> MGSSHHHHHHSSGPQQGLRQPQKEETKRPNIIFMMTDDHTTQAMSCYGGNLIQTPNMDRIANEGIRFDNCYAVNALSGPSRACILTGKFSHENGFTDNASTFNGDQQTFPKLLQQAGYQTAMIGKWHLISEPQGFDHWSILSGQHEQGDYYDPDFWEDGKHIVEKGYATDIITDKAINFLENRDKNKPFCMMYHQKAPHRNWMPAPRHLGIFNNTIFPEPANLFDDYEGRGKAAREQDMSIEHTLTNDWDLKLLTREEMLKDTTNRLYSVYKRMPSEVQDKWDSAYAQRIAEYRKGDLKGKALISWKYQQYMRDYLATVLAVDENIGRLLNYLEKIGELDNTIIVYTSDQGFFLGEHGWFDKRFMYEECQRMPLIIRYPKAIKAGSTSSAISMNVDFAPTFLDFAGVEVPSDIQGASLKPVLENEGKTPADWRKAAYYHYYEYPAEHSVKRHYGIRTQDFKLIHFYNDIDEWEMYDMKADPREMNNIFGKAEYAKKQK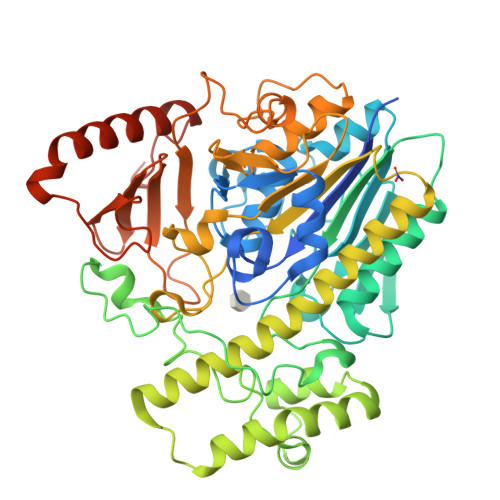ELMQLLEETQKQYKDNDPDEKETVLFKGDRRLMENR1H-indole-4-carboxamide | C9 H8 N2 O | 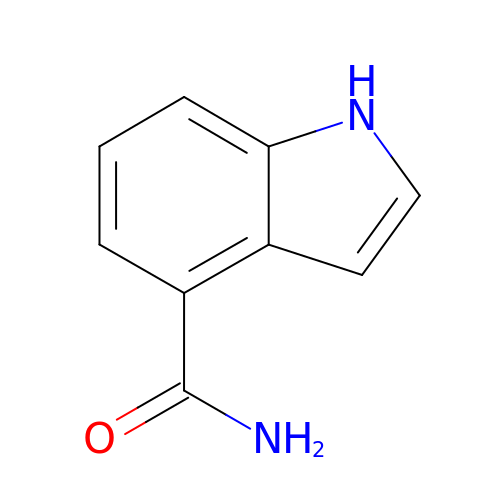ACRGIRLCXXEJCS-UHFFFAOYSA-N> MDG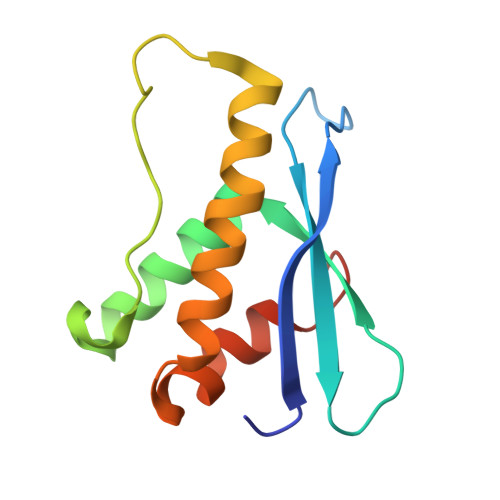RIKEVSVFTYHKKYNPDKHYIYVVRILREGQIEPSFVFRTFDEFQELHNKLSIIFPLWKLPGFPNRMVLGRTHIKDVAAKRKIELNSYLQSLMNASTDVAECDLVCTFFHGSHHHHHH>[2x]CGCGACC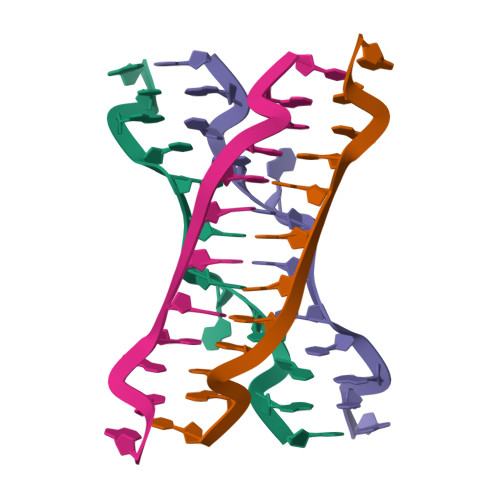TCGCG> QENRLLNESESSSQGLLGYYFSDLNFQAPMVVTSSTTGDLSIPSSELENIPSENQYFQSAIWSGFIKVKKSDEYTFATSADNHVTMWVDDQEVINKASNSNKIRLEKGRLYQIKIQYQREDPTEKGLDFKLYWTDSQNKKEVISSDNLQLPELKQKSSNSLEVLFQGSTSAGPTVPDRDNDGIPDSLEVEGYTVDVKNKRTFLSPWISNIHEKKGLTKYKSSPEKWSTASDPYSDFEKVTGRIDGNVSPEANHPLVAAYPIVHVDMENIILSKNEDQSTQNTDSQTRTISKNTSTSRTHTSEVHGNAEVHASFFDIGGSVSAGFSNSNSS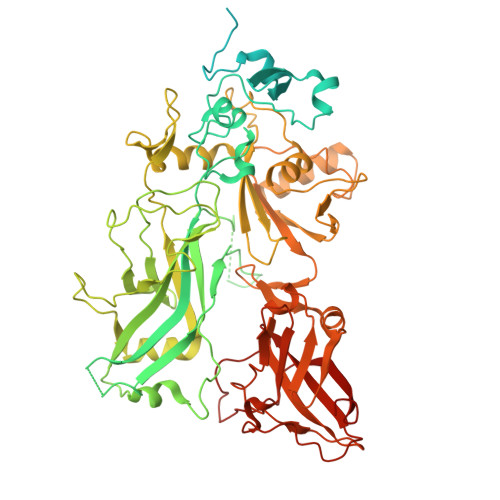TVAIDHSLSLAGERTWAETMGLNTADTARLNANIRYVNTGTAPIYNVLPTTSLVLGKNQTLATIKAKENQLSQILAPNNYYPSKNLAPIALNAQDDFSSTPITMNYNQFLELEKTKQLRLDTDQVYGNIATYNFENGRVRVDTGSNWSEVLPQIQETTARIIFNGKDLNLVERRIAAVNPSDPLETTKPDMTLKEALKIAFGFNEPNGNLQYQGKDITEFDFNFDQQTSQNIKNQLAELNATNIYTVLDKIKLNAKMNILIRDKRFHYDRNNIAVGADESVVKEAHREVINSSTEGLLLNIDKDIRKILSGYIVEIEDTEGLKEVINDRYDMLNISSLRQDGKTFIDFKKYNDKLPLYISNPNYKVNVYAVTKENTIINPSENGDTSTNGIKKILIFSKKGYEIG> GAMGSWNPKYDTRTLWTTPDTSPNCTIAQDKDSKLTLVLTKCGSQILANVSLIVVAGKYHIINNKTNPKIKSFTIKLLFNKNGVLLDNSNLGKAYWNFRSGNSNVSTAYEKAIGFMPNLVAYPKPSNSKKYARDIVYGTIYLGGKPDQPAVIKTTFNQETGCEYSITFNFSWSKTYENVEFETTSFTFSYIAQE;> MADFARSLSITTPEEMIEKAKGETAYLPCKFTLSPEDQGPLDIEWLISPADNQKVDQVIILYSGDKIYDDYYPDLKGRVHFTSNDLKSGDASINVTNLQLSDIGTYQCKVKKAPGVANKKIHLVVLGK

To date, all Ads display a characteristic, icosahedral symmetry in which 240 subunits of the trimeric hexon protein form the facets and 12 copies of the penton, comprising the pentameric penton base protein and the externally projecting trimeric fiber, form the vertices. At least in vitro and for most cell types, the fiber mediates the initial attachment to primary receptors, such as the D1 domain of the coxsackievirus and adenovirus receptor (CAR), sialic acids, CD46, and others (for review see Zhang & Bergelson). Our results showing that the CAV-2 fiber head contains a sialic acid binding site creates a paradox: both HAd37 and CAV-2 fiber heads contain CAR and sialic acid binding sites - but HAd37 uses sialic acid and CD46, while CAV-2 uses CAR (CAV-2 does not use CD46 to infect cells, unpublished data) to infect cells. We show by structural analysis that the CAV-2 fiber head also contains a sialic acid binding site, but in contrast to HAd37 this site is modestly involved in hemagglutination.

Among the HAds, serotype 37 is unusual: its fiber head can bind CAR, CD46 and sialic acid, but the virus appears to use only the latter two as functional receptors. To determine if sialic acid and CAR binding were mutually exclusive, we soaked CAV-2 or HAd37 fiber head crystals in complex with CAR in solutions containing sialyl-D-lactose. Crystals containing the complex with HAd37 fiber head diffracted to 1.55 Å and contained one chain of fiber head in complex with one CAR D1 molecule and one sialyl-D-lactose molecule in the asymmetric unit (space group I23). For both structures the electron density maps showed clear density for sialic acid, but not lactose, at the expected positions on the fiber heads. The HAd37 sialic acid binding site consists of three residues forming hydrogen bonds (Tyr213, Pro317 and Lys345) and two residues contacting sialic acid in hydrophobic interactions (Tyr308 and Val322). Burmeister et al. found that the sialic acid moiety bound to a basic patch close to the center of the trimeric fiber heads of HAd37 and HAd19p. Our results demonstrate that HAd37 interaction with human erythrocytes is primarily due to sialic acid binding via a conserved sialic acid binding site on this subgroup D HAd fiber head. In addition, although HAd37 head also binds CAR, in the context of the virus it does not appear to use CAR as a receptor, possibly due to its relatively short fiber.Elp3 acts as the catalytic subunit, but the loss of any of the six subunits results in hypo-modified U34 tRNAs in yeast, indicating that the complete integrity of the complex is important for its function. The enzymatically active Elp3 subunit of Elongator contains two functional domains, utilizes multiple cofactors, and conducts a unique uridine base modification specifically found only at the wobble base position of tRNAs. The two domains form a cleft that contains several highly conserved basic residues, which bind and accommodate the tRNA anticodon stem loop (ASL). The current model of a radical based Elp3-mediated cm5-modification reaction is proposed as follows (i) Elp3 recruits SAM and cleaves it to generate a 5’deoxyadenosine radical (5’-dA) in the rSAM domain, (ii) Elp3 hydrolyzes acetyl-CoA in the KAT domain and (iii) an acetyl radical is formed by the products of the two domains and (iv) is transferred onto the C5 position of U34 in the bound tRNA molecule.

We used full length and truncated versions of purified MinElp3 in crystallization trials and obtained well-diffracting crystals for monomeric MinElp3Δ1–19, MinElp3Δ1–46, and MinElp3Δ1–54. We solved their structures using a poly-alanine model of DmcElp3 via molecular replacement at 1.9 Å, 1.9 Å, and 2.1 Å resolution, respectively. Although all three versions contained various lengths of the N-terminus and also showed no signs of degradation, we could observe interpretable electron density only starting from residue V72 in all collected and refined datasets. Therefore, we believe that the N-terminus adopts a highly flexible conformation in the absence of substrate tRNAs. The main difference relates to the Fe–S cluster loop region (aa 87–123) and the Fe–S cluster itself, which were both completely unstructured in all monomeric MinElp3s. In our MinElp3 structures, we could not locate any bound Zn-ions and instead observed the formation of a disulfide bond between C384 and C389. In addition, we observed that the acetyl-CoA blocking loop (aa 466–486) is positioned outside of the acetyl-CoA binding pocket, interacting with the last visible residues of the N-terminus and also contacting a neighboring symmetry mate. We have previously reported that the ASL of (Dmc)tRNAGluUUC is not sufficient to bind to bacterial DmcElp3. In agreement with this data and the described importance of the extended N-terminus in MinElp3, we observed that the central basic cleft of MinElp3 is not sufficient for efficient ASL binding. The affinity between the truncated MinElp3Δ1–46 protein and the ASL alone are comparable to the one of an unspecific polyU sequence towards full length MinElp3. The first 45 residues seem to have a particularly strong contribution to the binding and deletion of the complete N-terminus resulted in affinities comparable to DmcElp3.

> GAMASNSEILKYATEEEKKILIPILRKKPVRTISGVAVVAVMTSPAKCPHGKCIFCPGGLDSVFGDVPQSYTGREPATMRGLMFNFDPYLQTRARIEQLEKVGHPTDKIELIIMGGTFPAREIEYQDWFIKRCLDAMNERESKSLEEAQKINETAKHRCVALCIETRPDYCSEKEINQMLKLGATRVELGVQSIYNEILKLCKRGHSVEDTIKATQLLKDSGLKVSYHLMPGMPGSSIEMDKKMFKEIFTNPDFMPDMVKIYPCLVIEGTELYEMWKRGEFKPYREEEAIEVISYAKSIMPKWVRTSRIQRDIPATVIVDGVKKSNLGELVYKYMEKKGLRCRCIRCREVGHVYYKKGILPDPEHIKLVREDYEASGGTEIFLSFEDVKNDILIAFLRLRDPYKPFRKEIDDKTMLVRQLHVFGWEKALTRDIKEVSWQHMGYGRMLMKEAERIAKEEFGKKKILVTSGIGVREYYRKLGYKRVGAYMGKEL>[4x]MRGLTVNFERINPMTNQTASTAKAMTAAEARAVADRAAAGFAGWSVLGPNARRAVLMKAAAALEARKDDFVQAMMAEIGATAGWAMFNLMLAASMIREAAALTTQIG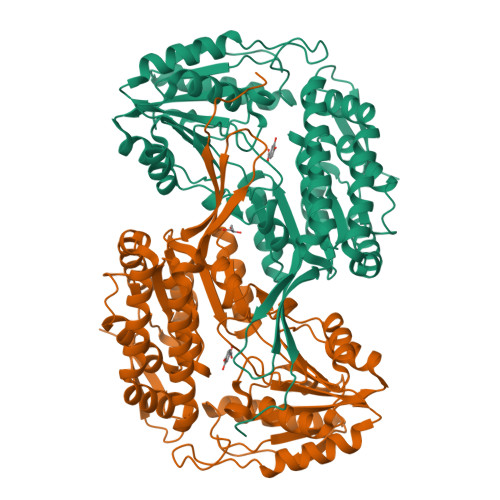GEVIPSDKPGCLALALREPVGVVLGIAPWNAPIILGVRAIAVPLACGNAVILKASEICPRTHGLIIESFAEAGFPEGVVNVVTNAPQDAGEVVGALIDHPAVKRINFTGSTGVGRIIAKRAAEHLKPCLLELGGKAPLVVLDDADLDEAAKAAAFGAFMNQGQICMSTERIIVVEAIAAEFTRRFAAKAQSMATGDPREGKTPLGAVVDRKTVDHVNTLIDDATAKGARIIAGGKGDSVLMSATVVDGVTAAMKLYRDESFGPIVGIIRAKDEADAVRLANDSEYGLAAAVFTRDTARGLRVARQIRSGICHINGPTVHDEAQMPFGGVGASGYGRFGGKAGIDQFTELRWITMETQPGHFPI> GAMGAWKLQTVLEKVRLSRHEISEAAEVVNWVVEHLLRRLQGGESEFKGVALLRTGSYYERVKISAPNEFDVMFKLEVPRIQLEEYCNSGAHYFVKFKRNPGGNPLEQFLEKEILSASKMLSKFRKIIKEEIKNIEDTGVTVERKRRGSPAVTLLISKPKEISVDIILALESKSSWPASTQKGLPISQWLGAKVKNNLKRQPFYLVPKHAKEGSGFQEETWRLSFSHIEKDILKNHGQSKTCCEIDGVKCCRKECLKLMKYLLEQLKKKFGNRRELAKFCSYHVKTAFFHVCTQDPHDNQWHLKNLECCFDNCVAYFLQCLKTEQLANYFIPGVNLFSRDLID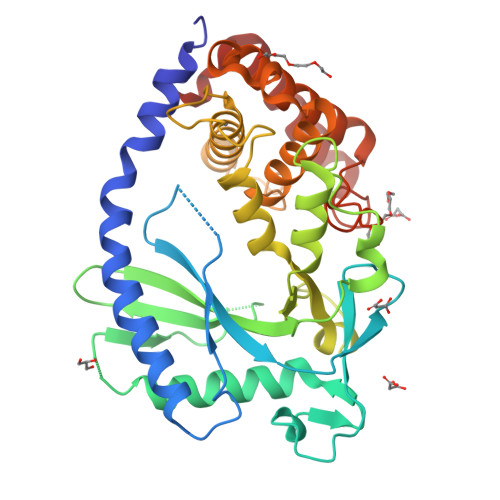KPSKEFLSKQIEYERNNGFPVFW>GPMGQKGWKFQGEQGEFRLEQPEHNSYLYFPLVNEAGMMSAVTPNLHGEITSGHNTFLMEPVSAESLHNSKASRNFWVFIEGYGAWSVSGNSARQNAARFTGEEERSAVEAGFLWHAVTRENEKAGLKARTVSFVPVTDDKIELMRVTLTNTGNAPLKLTPTAAIPLYGRSADDLRDHRHVTSLLHRIFTSEYGIEVQPALSFDERGHRVNKVTYGVFGAEAGGTAPAGFFPVTEDFIGEGGALDWPEAVVANREPDAQAGTAVEGYEAVGALRFAPVELAPGKSVSYVVAMVISGDRIDVGRYAADYLAAGRFDALLEQNRAYWRDKLDTVRFSSGDGEQDLWMKWVTLQPILRRLYGNSFLPYHDYGRGGRGWRDLWQDCLALMVMEPAEVRHLLLNNYAGVRMDGSNATIIGAGPGEFVADRNNIPRVWMDHGAWPLMTTLLYLHQSGDLDLLFQPQSYFRDVFVKRCRERDASWTPEQGNKLLTADGQIYEGTILEHILLQNIVPFFNVGEHGNIKLEGADWNDGLDLAPERGESVAFTAFYASNLMELSELLLELQKRTGKDSLDIAEEMALLLDTLGKPISYDSIQEKRSLLDRYYDAVTPRVSGKKLLLDIRKVAEDLKRKADWAVAHLRGSEWIQSKEGYAWFNGYYNNDGERVEGDHPDGVRMTLTGQVFAIMGGVATDEQTEKISQAVNRYLKDERIGYRLNSRFGGIQQNLGRAFGFAFGHKENGAMFSHMTVMYANALYKRGFVQEGFEVLDSIYRLSADFENSRIYPGVPEYINERGRGMYTYLTGSASWLLLTQLTEVYGVKGRFGDLRLEPKLVQAQFDGSGEAAVETLFAGRMLRVVYRNPQAAEHGQYRVDSVSLNGQSVDCQNDG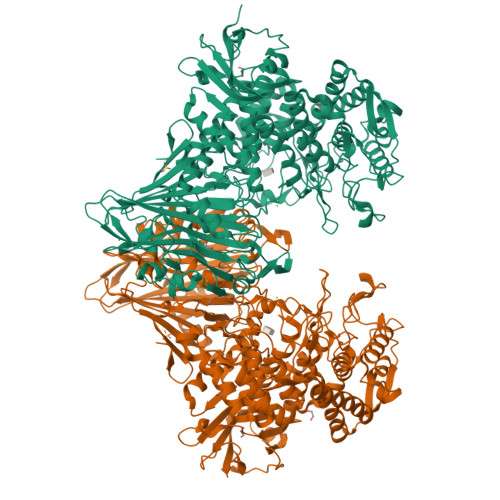AGCLIGRSLIEALPADGVHELIVTLGRNIS[2x]DIMETHYLAMINE 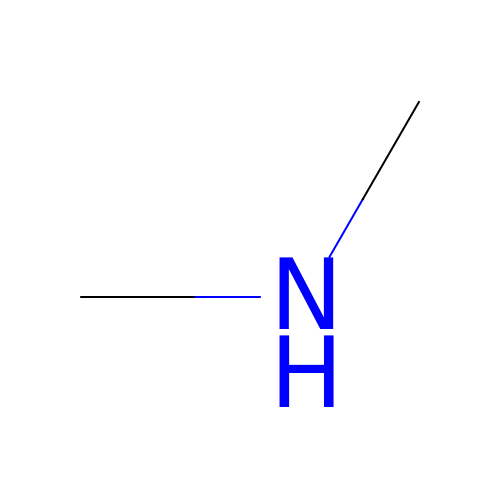| C2 H7 N | ROSDSFDQCJNGOL-UHFFFAOYSA-N>GSFTSNATNSNSAEKQRKIEESSRFADAVLDQYIGSIHSLCKDQHGCRFLQKQLDILGSKAADAIFEETKDYTVELMTDSFGNYLIQKLLEEVTTEQRIVLTKISSPHFVEISLNPHGTRALQKLIECIKTDEEAQIVVDSLRPYTVQLSKDLNGNHVIQKCLQRLKPENFQFIFDAISDSCIDIATHRHGCCVLQRCLDHGTTEQCDNLCDKLLALVDKLTLDPFGNYVVQYIITKEAEKNKYDYTHKIVHLLKPRAIE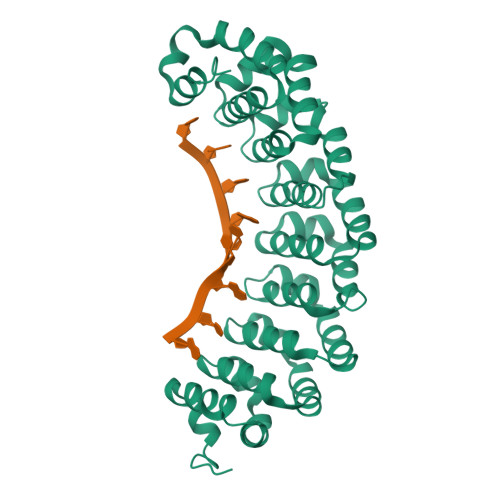LSIHKFGSNVIEKILKTAIVSEPMILEILNNGGETGIQSLLNDSYGNYVLQTALDISHKQNDYLYKRLSEIVAPLLVGPIRNTPHGKRIIGMLHLDS[2x]>[2x]RSIIGGKHGDRDVRILYQVGDSEEDLPVCAPNAVCSKIDLYETPWIERQCRCPDGRTCPSSLGVEDGHTIADKTRHYKMCQPVHKLPVCKHFRDYTWTLTTAAELNVTE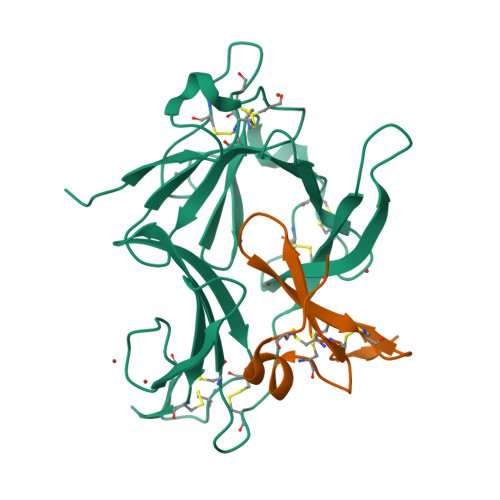QIVHCRCPRNSVTYLTKREPIGNDSPGYRYLFACSPLTRLRCQRKQPCKLFTVRKRQEFLDEVNINSLCQCPKGHRCPSHHTQSGVIAGESFLEDNIQTYSGYCMANDHHHHHH;>TFPTYKCPETFDAWYCLNDAHCFAVKIADLPVYSCECAIGFMGQRCEYKEID[2x]>VTDSINWASGEDDHVVARAEYDFAAVSEEEISFRAGDMLNLALKEQQPKVRGWLLASLDGQTTGLIPANYVKILGKRKGRKTV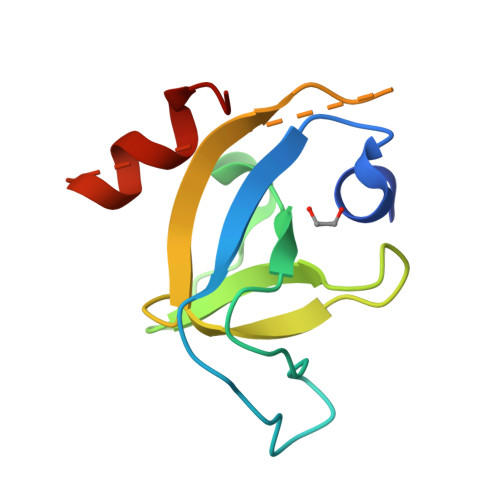ESSGGGGSGGGGSDEQEAAFESVFVE[2x]> MSGLSDFFTQLGQDAQLMEDYKQNPEAVMRAHGLTDEQINAVMTGDMEKLKTLSGDSSYQSYLVISHG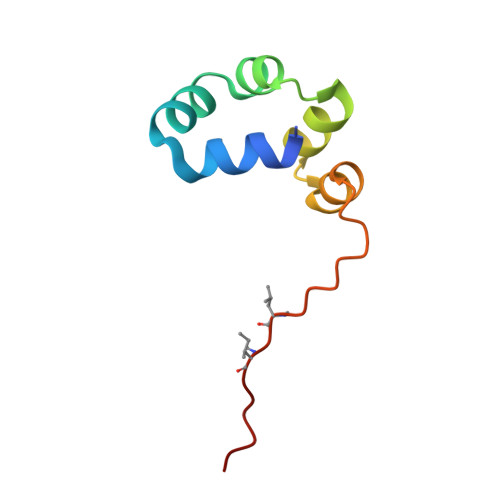NGD> VVRVADTMPSGPSNSESIPALTAAETGHTSQVVPSDTIQTRHVRNFHVRSESSVENFLSRSACVYIVEYKTRDDTPDKMYDSWVINTRQVAQLRRKLEFFTYVRFDVEVTFVITSVQDDSTRQNTDTPALTHQIMYVPPGGPIPQAVDDYNWQTSTNPSVFWTEGNAPPRMSIPFMSVGNAYSNFYDGWSHFSQTGVYGFNTLNNMGKLYFRHVNDKTISPITSKVRIYFKPKHVKAWVPR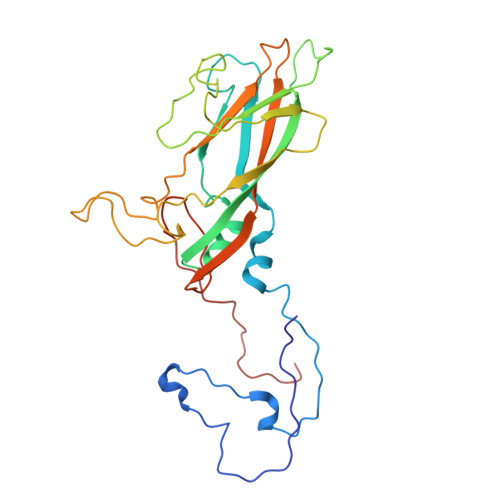PPRLCEYTHKDNVDFEPKGVTTSRTQLTISNS> GCFGRKMDRIS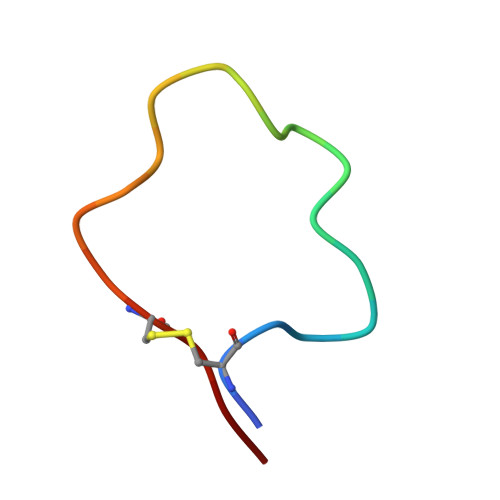SSSGLGCKVL>[2x]MGSSHHHHHHSSGLVPRGSPSASKVYKASDSAEAIEAFQLTPQQQHLIREDCQNQKLWDEVLSHLVEGPNFLKKLEQSFMCVCCQELVYQPVTTECFHNVCKDCLQRSFKAQVFSCPACR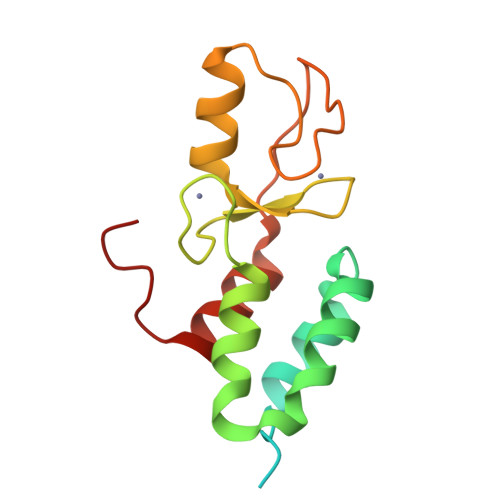HDLGQNYIMIPNEILQTLLDLFFPGYSKGR5-(4-azanylpiperidin-1-yl)carbonyl-1~{H}-pyridin-2-one | C11 H15 N3 O2 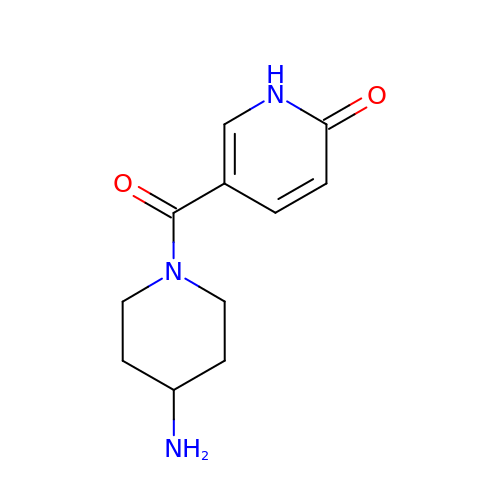| PBJCAAQZCVURJN-UHFFFAOYSA-N>[4x]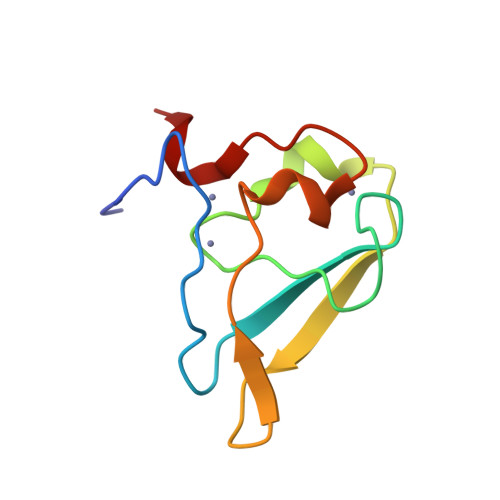GSVHKHTGRNCGRKFKIGEPLYRCHECGCDDTCVLCIHCFNPKDHVNHHVCTDICTEFTSGICDCGDEEAWNSPLHCKAEEQ;> RRAA> GMSHASFNSMFTYFQEPPFPDLLPPPPPPPYQRPLTLVITLEDFLVHSEWSQKHGWRTAKRPGADYFLGYLSQYYEIVLFSSNYMMYSDKIAEKLDPIHAF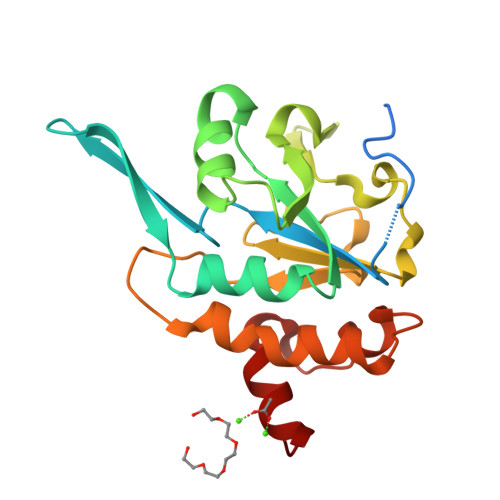VSYNLFKEHCVYKDGVHIKDLSKLNRDLSKVIIIDTDPNSYKLQPENAIPMEPWNGEADDKLVRLIPFLEYLATQQTKDVRPILNSFEDKKNLAEEFDHRVKK> GPELMVISRAEIYWADLGPPSGSQPAKRRPVLVIQSDPYNASRLATVIAAVITSNTALAAMPGNVFLPATTTRLPRDSVVNVTAIVTLNKTDLTDRVGEVPASLMHEVDRGLR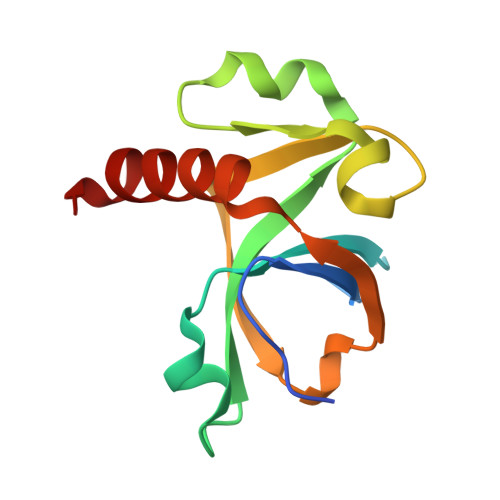RVLDL> MDSQRSTLVHWFRKGLRLHDNPALSHIFTAANAAPGRYFVRPIFILDPGILDWMQVGANRWRFLQQTLEDLDNQLRKLNSRLFVVRGKPAEVFPRIFKSWRVEMLTFETDIEPYSVTRDAAVQKLAKAEGVRVETHCSHTIYNPELVIAKNLGKAPITYQKFLGIVEQLKVPKVLGVPEKLKNMPTPPKDEVEQKDSAAYDCPTMKQLVKRPEELGPNKFPGGETEALRRMEESLKDEIWVARFEKPNTAPNSLEPSTTVLSPYLKFGCLSARLFNQKLKEIIKRQPKHSQPPVSLIGQLMWREFYYTVAAAEPNFDRMLGNVYCMQIPWQEHPDHLEAWTHGRTGYPFIDAIMRQLRQEGWIHHLARHAVACFLTRGDLWISWEEGQRVFEQLLLDQDWALNAGNWMWLSASAFFHQYFRVYSPVAFGKKTDPQGHYIRKYVPELSKYPAGCIYEPWKASLVDQRAYGCVLGTDYPHRIVKHEVVHKENIKRMGAAYKVNR

To compensate for this, archaea, prokaryotes and eukaryotes have photolyase proteins, which repair damaged DNA using the energy of visible light. The photoreceptor protein uses near-UV and visible light (300–500 nm) as an energy source to monomerize (6–4)TT [or (6–4)CC] lesions in DNA.

The cryo-structure reported in this paper increases the resolution to 1.79 Å. This is the highest resolution reported for Dm(6–4)PL in the PDB. Indeed, the mean r.m.s.d. calculated on the main-chain residues is 0.35 Å, which indicates that the position of the main chains was unchanged. Even the cryo-structure shows an unbent FAD. We conclude that the FAD is in a fully oxidized state in both of our structures. We therefore estimated the average diffraction-weighted X-ray dose during data acquisition to be approximately 3.2 MGy, which is a moderate dose in crystallography.>MSLMTAQIRLAEPADLNDDTLRARAVAAARGDQRFDVLITGGTLVDVVTGELRPADIGIVGALIASVHEPASRRDAAQVIDAGGAYVSPGLIDTHMHIESSMITPAAYAAAVVARGVTTIVWDPHEFGNVHGVDGVRWAAKAIENLPLRAIL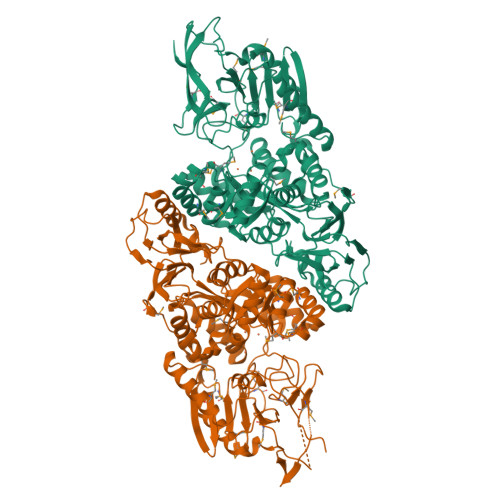LAPSCVPSAPGLERGGADFDAAILADLLSWPEIGGIAEIMNMRGVIERDPRMSGIVQAGLAAEKLVCGHARGLKNADLNAFMAAGVSSDHELVSGEDLMAKLRAGLTIELRGSHDHLLPEFVAALNTLGHLPQTVTLCTDDVFPDDLLQGGGLDDVVRRLVRYGLKPEWALRAATLNAAQRLGRSDLGLIAAGRRADIVVFEDLNGFSARHVLASGRAVAEGGRMLVDIPTCDTTVLKGSMKLPLRMANDFLVKSQGAKVRLATIDRPRFTQWGETEADVKDGFVVPPEGATMISVTHRHGMAEPTTKTGFLTGWGRWNGAFATTVSHDSHNLTVFGGNAGDMALAANAVIGTGGGMAVASEGKVTAILPLPLSGLVSDAPLEEVARAFEDLREAVGKVVEWQPPYLVFKACFGATLACNIGPHQTDMGIADVLTGKVMESPVIEVLGEGHHHHHH[2x]>MLVVPAIDLFRGKVARMIKGRKENTIFYEKDPVELVEKLIEEGFTLIHVVDLSNAIENSGENLPVLEKLSEFAEHIQIGGGIRSLDYAEKLRKLGYRRQIVSSKVLEDPSFLKSLREIDVEPVFSLDTRGGRVAFKGWLAEEEIDPVSLLKRLKEYGLEEIVHTEIEKDGTLQEHDFSLTKKIAIEAEVKVLAAGG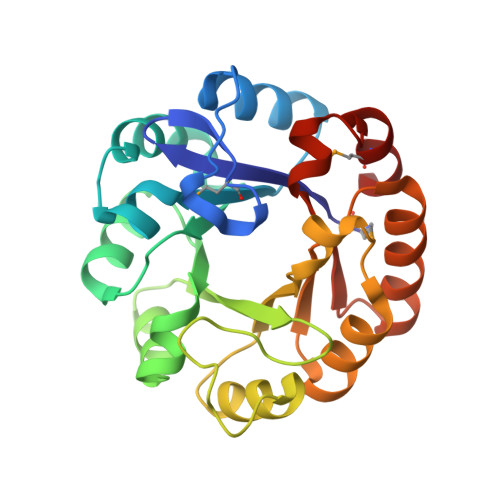ISSENSLKTAQKVHTETNGLLKGVIVGRAFLEGILTVEVMKRYAR[2x]Mutations in CK1δ/ε (hereafter referred to jointly as CK1), as well as PER2, exert powerful control over circadian period, altering the intrinsic timing of circadian rhythms by hours in vivo. PER2 is regulated by a CK1-dependent phosphoswitch, where kinase activity at two antagonistic sites functionally interact to control PER2 stability. We discovered a conformational switch in the activation loop of CK1 that regulates its activity on two regulatory regions in PER2 that control its stability and circadian timing in mammals. We show that anion binding regulates the conformation of this switch to reshape the substrate binding cleft and thereby control substrate selectivity.

Since the first structure of CK1δ published in 1996, nearly all CK1 structures have been determined after crystallization with high concentrations of sulfate or citrate anions. Because anion binding at Site two is incompatible with the activation loop in its ‘loop up’ conformation, prior crystallographic conditions have likely disfavored this alternate conformation. To determine if we could independently capture the two states of the activation loop switch in the native kinase, we optimized sulfate-free crystallographic conditions and solved a structure of anion-free CK1δ. Therefore, CK1 has an anion-dependent switch in its activation loop.

>[2x]MELRVGNRYRLGRKIGSGSFGDIYLGTDIAAGEEVAIKLECVKTKHPQLHIESKIYKMMQGGVGIPTIRWCGAEGDYNVMVMELLGPSLEDLFNFCSRKFSLKTVLLLADQMISRIEYIHSKNFIHRDVKPDNFLMGLGKKGNLVYIIDFGLAKKYRDARTHQHIPYRENKNLTGTARYASINTHLGIEQSRRDDLESLGYVLMYFNLGSLPWQGLKAATKRQKYERISEKKMSTPIEVLCKGYPSEFATYLNFCRSLRFDDKPDYSYLRQLFRNLFHRQGFSYDYVFDWNMLK> RKLCSLDNGDCDQFCHEEQ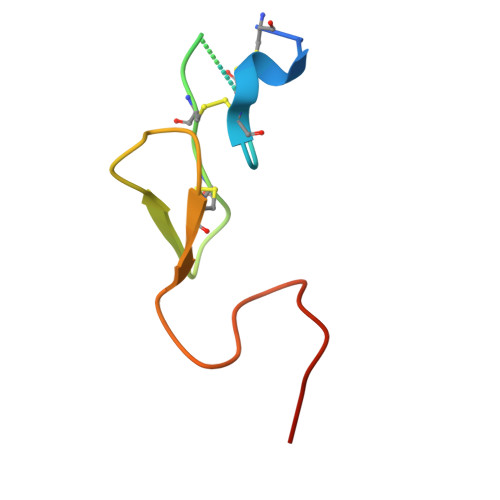NSVVCSCARGYTLADNGKACIPTGPYPCGKQTLERR> MVLEMLNPIHYNITSIVPEAMPAATMPVLLLTGLFLLVWNYEGTSSIPGPGYCMGIGPLISHGRFLWMGIGSACNYYNRVYGEFMRVWISGEETLIISKSSSMFHIMKHNHYSSRFGSKLGLQCIGMHEKGIIFNNNPELWKTTRPFFMKALSGPGLVRMVTVCAESLKTHLDRLEEVTNESGYVDVLTLLRRVMLDTSNTLFLRIPLDESA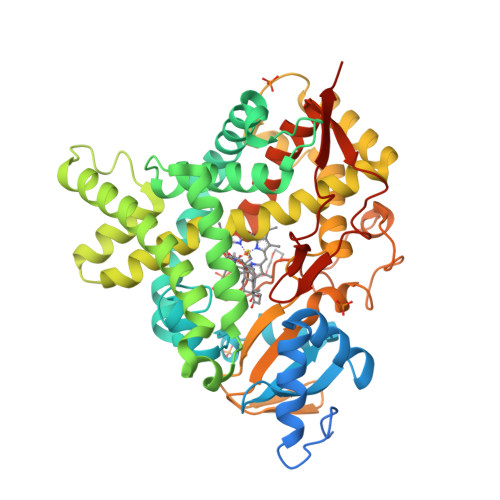IVVKIQGYFDAWQALLIKPDIFFKISWLYKKYEKSVKDLKDAIEVLIAEKRRRISTEEKLEECMDFATELILAEKRGDLTRENVNQCILEMLIAAPDTMSVSLFFMLFLIAKHPNVEEAIIKEIQTVIGERDIKIDDIQKLKVMENFIYESMRYQPVVDLVMRKALEDDVIDGYPVKKGTNIILNIGRMHRLEFFPKPNEFTLENFAKNVPYRYFQPFGFGPRGCAGKYIAMVMMKAILVTLLRRFHVKTLQGQCVESIQKIHDLSLHPDETKNMLEMIFTPRNSDRCLEH> MSKHELSLVEVTHYTDPEVLAIVKDFHVRGNFASLPEFAERTFVSAVPLAHLEKFENKEVLFRPGFSSVINISSSHNFSRERLPSGINFCDKNKLSIRTIEKLLVNAFSSPDPGSVRRPYP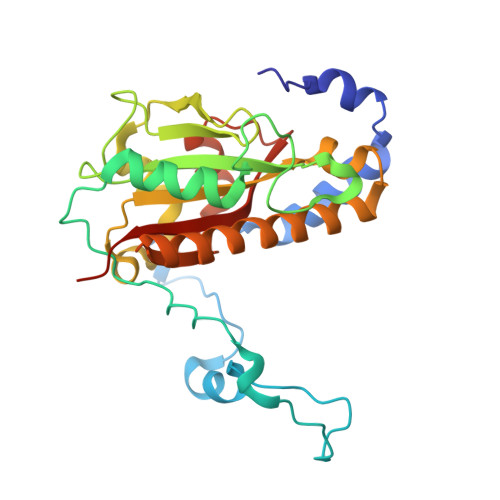SGGALYPIEVFLCRLSENTENWQAGTNVYHYLPLSQALEPVATCNTQSLYRSLSGGDSERLGKPHFALVYCIIFEKALFKYRYRGYRMALMETGSMYQNAVLVADQIGLKNRVWAGYTDSYVAKTMNLDQRTVAPLIVQFFGDVNDDKCLQ>MAPSLDSISHSFANGVASAKQAVNGASTNLAVAGSHLPTTQVTQVDIVEKMLAAPTDSTLELDGYSLNLGDVVSAARKGRPVRVKDSDEIRSKIDKSVEFLRSQLSMSVYGVTTGFGGSADTRTEDAISLQKALLEHQLCGVLPSSFDSFRLGRGLENSLPLEVVRGAMTIRVNSLTRGHSAVRLVVLEALTNFLNHGITPIVPLRGTISASGDLSPLSYI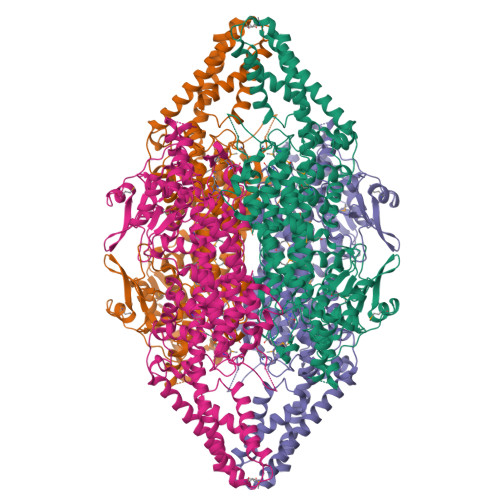AAAISGHPDSKVHVVHEGKEKILYAREAMALFNLEPVVLGPKEGLGLVNGTAVSASMATLALHDAHMLSLLSQSLTAMTVEAMVGHAGSFHPFLHDVTRPHPTQIEVAGNIRKLLEGSRFAVHHEEEVKVKDDEGILRQDRYPLRTSPQWLGPLVSDLIHAHAVLTIEAGQSTTDNPLIDVENKTSHHGGNFQAAAVANTMEKTRLGLAQIGKLNFTQLTEMLNAGMNRGLPSCLAAEDPSLSYHCKGLDIAAAAYTSELGHLANPVTTHVQPAEMANQAVNSLALISARRTTESNDVLSLLLATHLYCVLQAIDLRAIEFEFKKQFGPAIVSLIDQHFGSAMTGSNLRDELVEKVNKTLAKRLEQTNSYDLVPRWHDAFSFAAGTVVEVLSSTSLSLAAVNAWKVAAAESAISLTRQVRETFWSAASTSSPALSYLSPRTQILYAFVREELGVKARRGDVFLGKQEVTIGSNVSKIYEAIKSGRINNVLLKMLA[2x]>[2x]MIDINLIREKPDYVKERL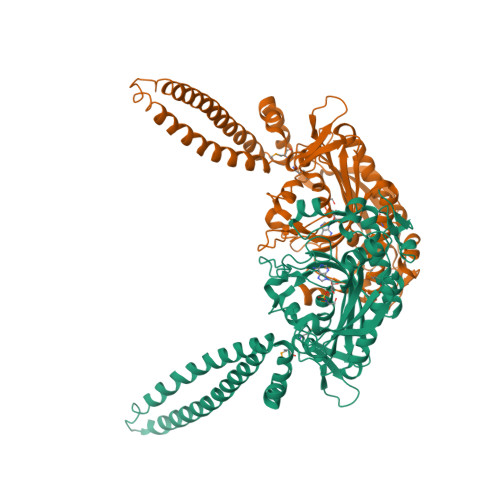ATRDKELVSLVDKVLELDKRRREIIKRLEALRSERNKLSKEIGKLKREGKDTTEIQNRVKELKEEIDRLEEELRKVEEELKNTLLWIPNLPHPSVPVGEDEKDNVEVRRWGEPRKFDFEPKPHWEIGERLGILDFKRGAKLSGSRFTVIAGWGARLERALINFMLDLHTKKGYKEICPPHLVKPEILIGTGQLPKFEEDLYKCERDNLYLIPTAEVPLTNLYREEILKEENLPIYLTAYTPCYRREAGAYGKDIRGIIRQHQFDKVELVKIVHPDTSYDELEKLVKDAEEVLQLLGLPYRVVELCTGDLGFSAAKTYDIEVWFPSQNKYREISSCSNCEDFQARRMNTRFKDSKTGKNRFVHTLNGSGLAVGRTLAAILENYQQEDGSVVVPEVLRDYVGTDVIRPE>MTISRRDFLNGVALTIAAGLTPAEILRAAPGGRYYPPALTGLRGSHPGAFEVAHQMGWEKKTFDVDHLPIEEEYDLVVVGGGISGLAAAWFYRERHPAARILVIENHDDFGGHAKRNEFQAGGRTILGYGGSESLQSPNALYSEDAKHLLKRLGVELKRFETAFDTDFYPGLGLSRAVFFDKASFGVDKLVSGDPTPMVADEVPRDRLNARSWRAFIGDFPLSREDREALIALYESPR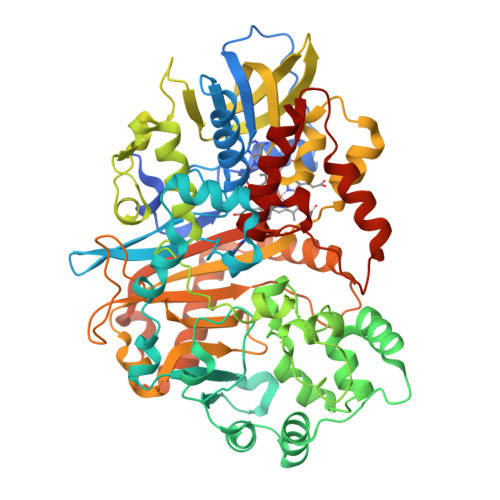DYLAGKSVEEKETYLAKTSYRDYLLKNVGLSETSVKYFQGRSNDFSALGADALPAADAYAAGFPGFDALGLPQPSEEAQAEMDEPYIYHFPDGNASLARLMVRDLIPAVAPGRGMEDIVMARFDYSKLDLAGHPVRLRLNSTAVSVRNRAGGVDVGYSRAGRLHRVRGKHCVMACYNMMVPYLLRDLSEEQAHALSQNVKFPLVYTKVLLRNWQAWKTLGIHEIYAPTLPYSRIKLDFPVDLGSYRHPRDPRQPIGVHMVYVPTTPNAGMDARTQARVGRSKLYAMSFEQLEKDIRDQLQAMLGPAGFDHRRDITGITVNRWSHGYSYFMNTLYDDEAESEALMELARSKVGNVAIANSDAAWDAYAHAAIDQAVRAVRELG[2x]> KVSSPKIQVYSHYPGEYGKENTLICYVSGFHPPDISIELLKNGEVIADAQQTDLAFEKGWQFHLTKSVSFKPEKSDEYSCSVRHMSKTKK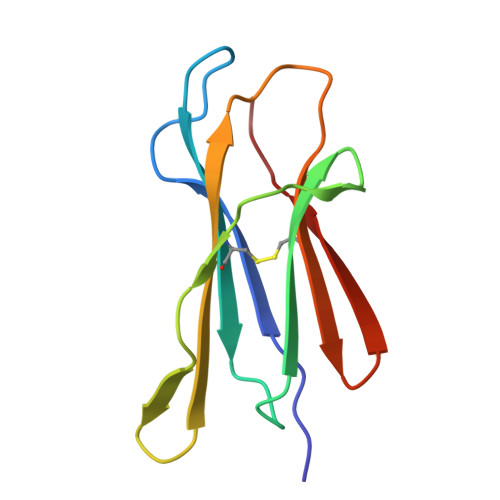IVWESNM> SDLPPVAKAAQVVNQTLQLDDSYPDLDSYCRPGASSDYEMQSSDSSWAPFHVVRHHNIPDKVFEHLNAGEVFTKLGLFAEIGYAWASIDSSLFLWDYTHPNPELIGYEEATHTITAVALVPPKPGVFVKTITHVLVVATTSEIILLGVSATPTPSGSKSLTLYSTRMSVHRGGSDVSFIVGTKDGRIFLGGESDTDIHEIFYQQEERWFSSRCGKINHSHPFGSRQQEWLRGLYVDDTRNLLYSLSNRSTIRTYHMEGPEKLTKVIEKDKTSCLRDFAHMADSSPLFTDKTNIVALSPIPATEASKLHLMALTDTGCRLFLSATSSASYTMGGATSLAPQSMQLQFVKFPPRESPTRIRTLNGQIIDSQLDKTSRALDPSALGFRFSPGYFFDVVRKHPNQDMLFVSAPDTGRIKVTQPASALKYFEQGTWIELENGNRTI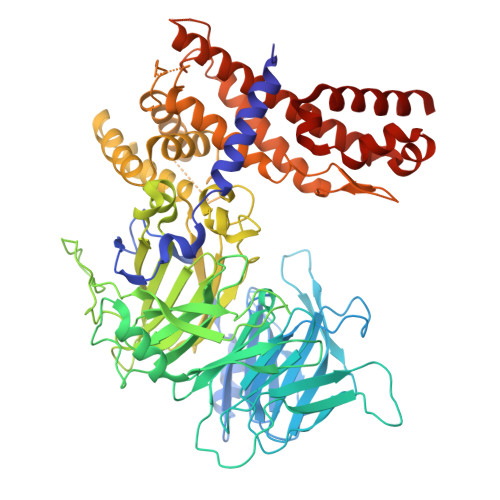EIGLTTAPFAAAKQPLGFGNELAVQFDQVPGEFAVLTNTGVHIVRRRRLVDIFAKALGNCVSASDDALEREVRKFINQYGRVETIAAALAVACGQGSDLRTGTGRGMDRNTENLARAAFIEYGGQPRLAESDGKQSVSESVRLSSRHDALALYLTRLVRTLWKAKVVQVGSGSDISSTIPTSKLVTIQENVERLRNFLEANKSTIQGLAPPSERLFGRQEDIANQKEHQALHALQKLMESISEGISFVLMLFDERVSDIYARLDAVSQQQLKDLTYEQLFSQTPGKELAKVLVKAIVNRNI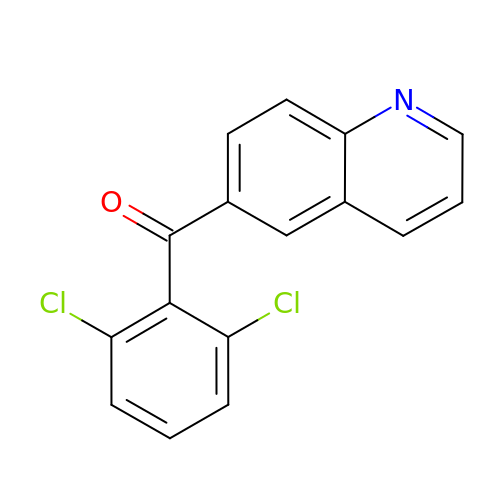(2,6-dichlorophenyl)(quinolin-6-yl)methanone | C16 H9 Cl2 N O | LMXZTTBPURRZTL-UHFFFAOYSA-N>[2x]MAGKKVLIVYAHQEPKSFNGSLKNVAVDELSRQGCTVTVS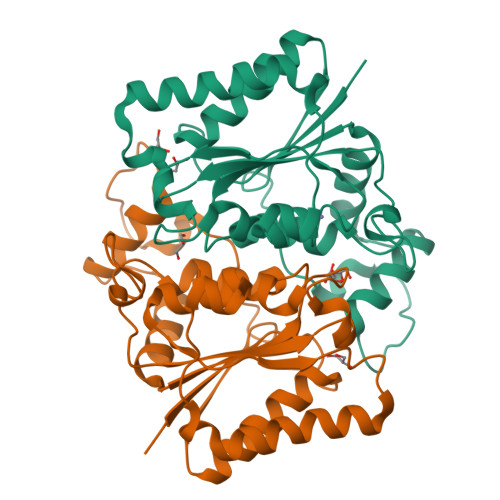DLYAMNFEPRATDKDITGTLSNPEVFNYGVETHEAYKQRSLASDITDEQKKVREADLVIFQFPLYWFSVPAILKGWMDRVLCQGFAFDIPGFYDSGLLQGKLALLSVTTGGTAEMYTKTGVNGDSRYFLWPLQHGTLHFCGFKVLAPQISFAPEIASEEERKGMVAAWSQRLQTIWKEEPIPCTAHWHFGQ>SMGTSPSSKYVKLNVGGALYYTTMQTLTKQDTMLKAMLSGRMEVLTDSEGWILIDRCGKHFGTILNYLRDGAVPLPESRREIEELLAEAKYYLVQGL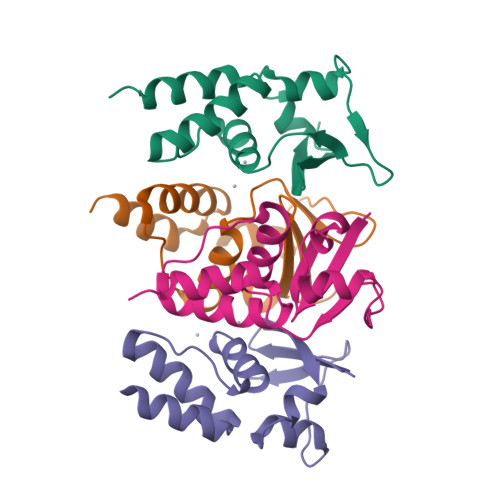VEECQAALQNKDTYE[4x]Cyclodipeptide synthases (CDPSs) are enzymes that use sequentially two aminoacyl-tRNAs (aa-tRNAs) to catalyze the formation of two peptide bonds leading to the production of various cyclodipeptides (Gondry et al. 2009; Canu et al. 2019). CDPSs are built around a Rossmann fold similar to the catalytic domain of the two class Ic aminoacyl-tRNA synthetases (aaRSs), TyrRS and TrpRS. Overall, the data show that the first aa-tRNA binds the enzyme with its aminoacyl moiety accommodated in a P1 pocket. Here, we study the binding of E. coli phenylalanyl-tRNAPhe (Phe-tRNAPhe) to the XYP-CDPS from Candidatus Glomeribacter gigasporarum (Cglo-CDPS) by gel filtration and electrophoretic mobility shift assay.

However, during the search for crystals containing Cglo-CDPS-S32A:Phe-tRNAPhe complex, we identified crystals containing only tRNAPhe. In a first step, we used these crystals to determine the structure of tRNAPhe overproduced in E. coli at 3.1 Å resolution. The structure of the overproduced E. coli tRNAPhe contains nucleotides 1 to 75. Among the 10 modified nucleosides of mature E. coli tRNAPhe, 3-(3-amino-3-carboxypropyl) uridine (acp3U) was visible at position 47. 4-thiouridine (S4U) at position 8, dihydrouridine (D) at positions 16 and 20, pseudouridine (ψ) at positions 32, 39, and 55 were also modeled because these modifications are isosteric with the original bases although, at 3.1 Å resolution, no further validation was available in the electron density map. Finally, 2-methylthio-N6-isopentenyladenosine (ms2i6A) at position 37, 7-methylguanosine (m7G) at position 46 were not modeled because the modifications were not visible in the electron density map. Comparison of the tRNAPhe structure with that of unmodified tRNAPhe shows that the two molecules are very close to one another (rmsd = 2.56 Å for 1572 atoms compared). In particular, both tRNAs harbor a G10–C25–G44 triplet base pair. U45 is flipped out of the tRNA core and forms Watson–Crick interactions with A26 of a symmetry-related molecule. Hence, in tRNAPhe, U45 may have a marked propensity to adopt the flipped-out conformation.

> GCCCGGAUAGCUCAGUCGGUAGAGCAGGGGAUUGAAAAUCCCCGUGXCCUUGGUUCGAUUCCGAGUCCGGGCACCA> TIHQHVDESQSSLHHTEKQIQTFITQHNNSFQELDLTNHHDVTATKRELLKLIHQQPATLYYELSGPNQFITNNYEHLNTKNMYLFSTHQLKFKNSTYMLKIYMANTPRLSEIKKDNRQFALIVD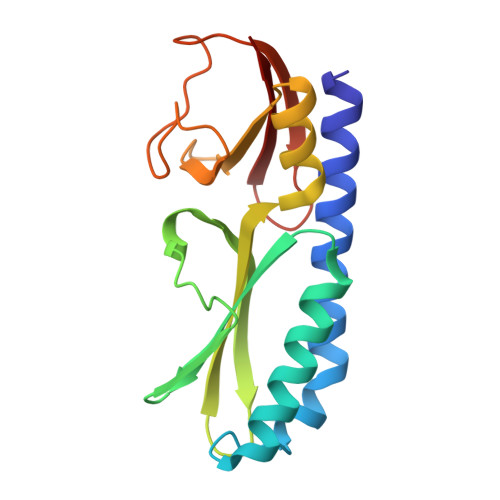QYDNILYANDDRFTIGEKYRPQQFGFMNESVKLNHADHRLIIYKDI>[2x]DVQTALQHSIREIGLRLMRMKNDGMSQKDIAAKEGLSQAKVTRALQAASAPEELVALFPVQSELTFSDYKTLCAVGDEMGNKNLEFDQLIQNISPEINDILSIEEMAEDEVKNKILRLITKE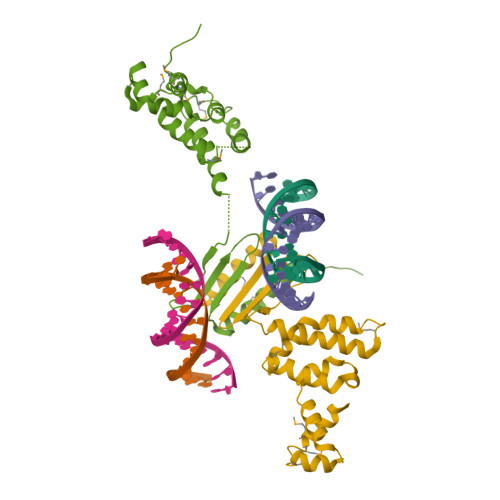ASLLTDKGSKDKSVVTELWKFEDKDRFARKRVKGRAFSYEFNRLSKELQEELDRMIGHILRKSLDKKPKP> MNNLKPFIYYDWKKTILKNAKESYSINEIIPKTFFMELHGTKITNSTLNGTWKAWNLTDEGEGSHPVLKCIIDDGYLDMNFGASSEKIPLKNVWIKLCMKINPNSDGTYSIPEKSSSFYIKDNSLKISKDNLILDKYLNKLMLSYFKNNIKNIEMFINKSRIQTKVVGDLSLLGWNTENSVSFRTMNEFIKKDNLYPKDFKAVYSYRKMTFTATGTFDSWEMTTGADGRNIRFKCPIKSAAYDLDGDVFNSSTENFLLIQVDLTYFDSKTTINDPTGENDGKQFNLKVKTNDDKLKNVLIVTYNLTDTDGSMSSEDKDFLSLAFRNWFNDNIQQFEQIFAYILLD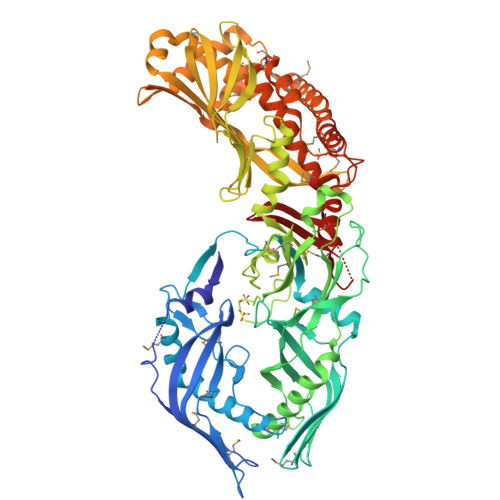ETAKIPEYQWLKPTQISYGSASVETANDEPDLDASIFSAMSMVENNTNSTPSHAVDNRMLQLTKTQAAFGISFPLFIEHFLKQALLSSQFISVDDIVADINTLTITNNKQIIFGKVENSDGKNVDSSLKPGKLKLSLQNNLIVLELFDLTWEQGRGVTGHFDFRQEYELTLESKSEKQIPILKVHDEPEIEYYVEEAQWKANEDMIVSAVVGTVFSMILGAGMKLAGSALSKAGKLIRSKATTIKGRKKIYINRSNVRQLRKDSGVTEMELQRINRRNSSIASEDARFISNNGTTSIQTLGDMKKKPMSTGQRIAIGVKKITGTAVMFGAVGLGMNFGEMLINYINAMENNDYSAIPGINSFMQQCIGAMQWPDKDSELKVTFGKLQGIYLLGGTLEKNNKPNSK>[2x]GPMEADIITNLRCRLKEAEEERLKAAQYGLQLVESQ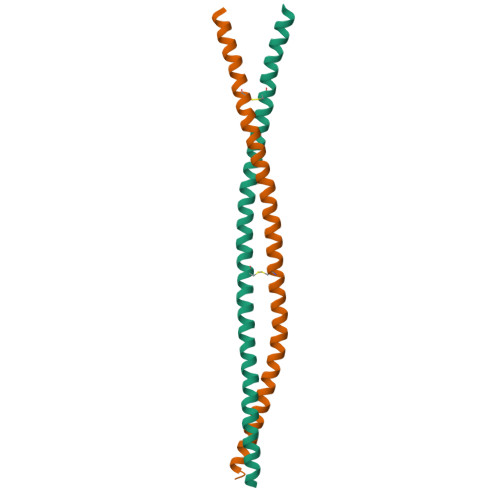NELQNQLDKCRNEMMTMTESYEQEKYTLQREVELKSRMLESLSCECEAIKQQQKMHLEKLEEQLSR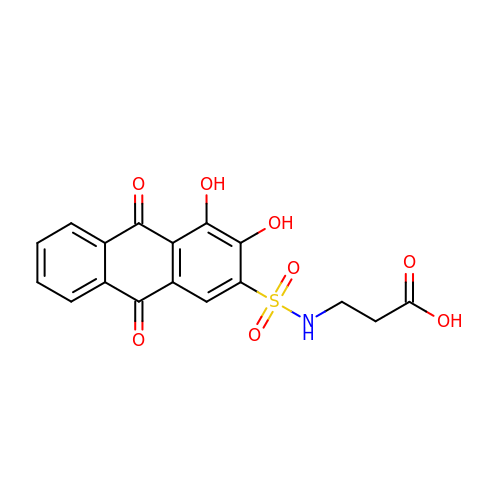N-(3,4-dihydroxy-9,10-dioxo-9,10-dihydroanthracene-2-sulfonyl)-beta-alanine | C17 H13 N O8 S | TVGDFUTTWNAYMD-UHFFFAOYSA-N>[4x]HHHHHHMETKENPWWKKAVVYQIYPKSFKDTTGNGVGDIRGIIEKLDYIKELACDVIWLTPIYQSPQNDNGYDISDYYSIHEEYGTMADFEELLEEAHKRGIKVIMDLVVNHTSTEHRWFKEAASGKENLYRDFYIWKDMKPNGAPPTNWESKFGGSAWEFHAESGQYYLHLYDVTQAD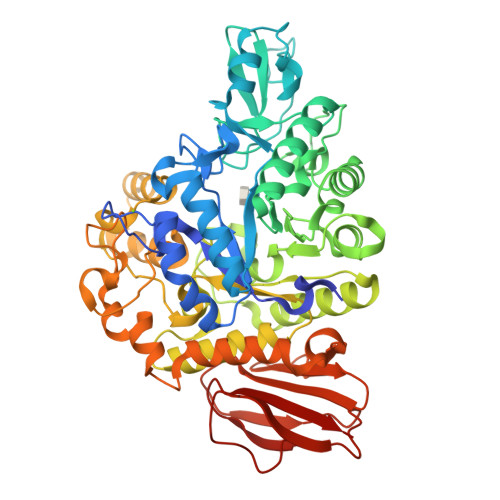LNWENEAVRKKVYEMMHFWFEKGIDGFQLDVINVISKDQRFPDDDEGDGRRFYTDGPRVHEFLNEMNREVFSKYDSMTVGEMSSTTIADCIRYTNPESRELDMVFNFHHLKADYPNGEKWALADFDFLKLKKILSEWQTEMNKGGGWNALFWCNHDQPRIVSRYGDDGKYRKKSAKMLATAIHMLQGTPYIYQGEELGMTNPKFDDISLYRDVESLNMYRILKEAGKPEAEIIEILKAKSRDNSRTPVQWNGEENAGFTAGTPWIPVPDNYKEINAEEALNDPDSIFYHYKKLNELRKEFDIITTGDYQLILEDDQELYAYLRNGADEKLLVINNFYGKETEFQLPDDIDIEGYDAKVLISNDTDLPESFKRFTVKPYQSIVYHLAKPC>[5x]MTSRKKVLLKVIILGDSGVGKTSLMNQYVNKKFSNQYKATIGADFLTKEVMVDDRLVTMQIWDTAGQERFQSLGVAFYRG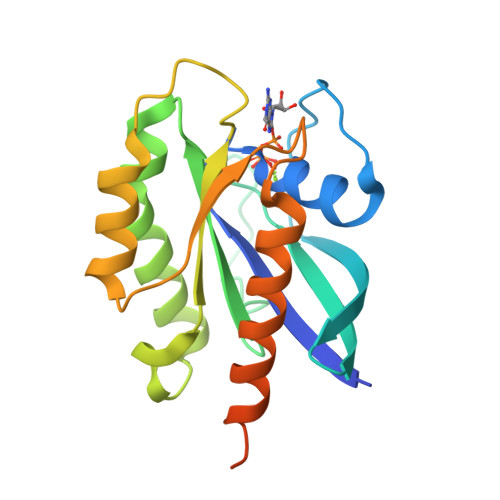ADCCVLVFDVTAPNTFKTLDSWRDEFLIQASPRDPENFPFVVLGNKIDFENRQVATKRAQAWCYSKNNIPYFETSAKEAINVEQAFQTIARNALKQETEVELYNEFPEPIKLDKNDRAKASAESCSC Processive pan-editing of multiple editing blocks within a single transcript is dependent on the 20-subunit RNA editing substrate binding complex (RESC) that serves as a platform to orchestrate the interactions between pre-mRNA, guide RNAs (gRNAs), the catalytic RNA editing complex (RECC), and a set of RNA helicases. Here we report the cryo-EM structure of Trypanosoma brucei RESC1–RESC2, a central hub module of the RESC complex. RESC1 and RESC2 form a complex and are dependent on each other for stability. Although the tertiary structures of both subunits closely resemble each other, only RESC2 selectively binds 5′-triphosphate-nucleosides, a defining characteristic of gRNAs.

We solved the cryo-EM structure of the complex and built the model into the final 3.4 Å resolution map with an AlphaFold prediction of the dimeric complex as a starting point. The final model comprises RESC1 residues 152–175 and 185-C, and RESC2 residues 133–161 and 171–483. For each subunit, a small N-terminal domain (RESC1 46–100 and RESC2 51–107) connected by a long linker (RESC1 101–151 and RESC2 108–132) is predicted by AlphaFold but not resolved in the final cryo-EM map, suggesting flexibility within the linker region. In the model, the tertiary structures of both subunits resemble each other, with an RMSD of 1.159 Å. Each subunit comprises an imperfect β-barrel composed of 10 β-strands that are surrounded by five α-helices. The inside of each barrel forms a tunnel that is accessible to solvent and possible ligands. The subunits dimerise through a domain-swapped β-harpin (two antiparallel β-sheets, β-2 and β-3, connected by a ca. 15 amino acid long loop). The dimerisation interface of the subunits provides a contact area of 2426 Å2 and involves about 28% of the resolved domain, as calculated by PDBePISA. In each subunit, a hydrophobic patch binds the β-harpin of the other subunit, mediated by interactions between β-2 and β-3 of the hairpin with β-4, β-5 and helix B of the barrel. Both β-hairpins carry hydrophobic residues for binding to the surface of the barrel, but their connection loops differ in sequence and chemical properties: the loop of RESC2 contains charged residues (K195, Q199, K201, N204) that interact with the surface of RESC1, while the loop of RESC1 contains hydrophobic residues (V173, F178, F181). The RESC1 hairpin is more flexible, indicated by the lower map quality that did not allow model building for this loop. These differences in the domain swap configuration rationalise the preference for RESC1–RESC2 heterodimerisation rather than homodimerisation and the instability of the subunits when expressed alone.

> MKHHHHHHSAGLEVLFQGPDSMQNQGSVSQGALNMRDQQAAAAENVTPERVWALWNEGNLFSLSLAQLQGFLSRCGVRTDPAAKKAAVVRQVEEYLHSKDTTVKGGGQGAASPQQHQQHGQQGGYGRWNQASVMQPETLLDLSQAGFYEGAANMVPKAFQLLVSDTAPDVVVSRVNTTAFPGFPSNTECYTLGASEKDVAIRSRYSKVLQWCCLNMSNLQMDGELYVDFGKLLLKPSVMRKNRRIVSSYTLQQRLQVNHPYTWVPTLPESCLSKIQEQFLQPEGFAPIGKGVQLTYSGTIKRSKDQLHVDLDNKGKVLAVNSAWVNLQTAWCTHAKGPDVRLLLRSRPPIRRQDVELFASTPIIKLADDDVADVLPPEHGQLVYLSEDETRLFERVSDRGVTITVREVKRQPLIILRDEEEDPRVEYSLSAHIPANAAKATDVRAVGLTAFELAGRLAGLVAEDFVREYGCEAKL;> MQSFSAAAPAASGDFSHITRNTVWGLWNEGNLFSLSVPELAFFLQEHCRVANVDPRAKKSALVRQVEEILSAEQQASATVPQEDNPHAIVVTDYDRAEDALEEADEYGDWGAEPGFEDRRELDFMELSPGRMGERYDPLSPRAFQLLHSETATDVGIASIDPSKLPGQSKVKNALAAIHVAPNDANKMRFRMAFEWCLMNIWNMNMPGELNIGAGKALYYRSVAKQNRNVMPLWTVQKHLYAQHPYAWFAIASESNVAAMESLAAALNMSIQQERTTSYKVTIRRMAEFFDCELNGQLKCTMMNKPWDRFFVSHYIRSKMPDLRYVVRARHPIKKRIADAYLEADILRSTRDSVQSVLSPELGDVVYCCERVVRKWAKKTATGVTLQLVETKRTPLIITKAGDEGERLEYEWIVPLPQQAERIDIAALTDELWEYGNKLAAALEEGMEELMVHTMTAVSAY>MVGYSSKLIFVSMITRHGDRAPFANIENANYSWGTELSELTPIGMNQEYNLGLQLRKRYIDKFGLLPEHYVDQSIYVLSSHTNRTVVSAQSLLMGLYPAGTGPLIGDGDP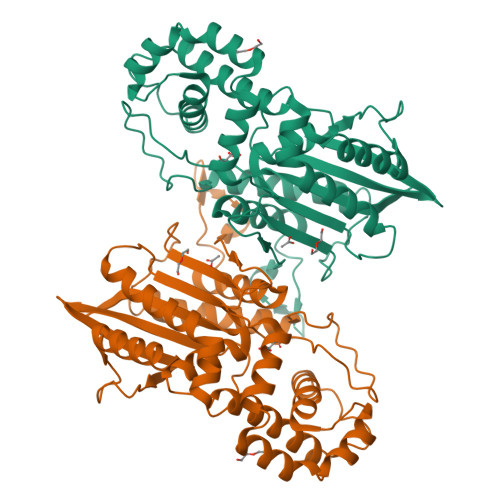AIKDRFQPIPIMTLSADSRLIQFPYEQYLAVLKKYVYNSPEWQNKTKEAAPNFAKWQQILGNRISGLNDVITVGDVLIVAQAHGKPLPKGLSQEDADQIIALTDWGLAQQFKSQKVSYIMGGKLTNRMIEDLNNAVNGKSKYKMTYYSGHDLTLLEVMGTLGVPLDTAPGYASNLEMELYKDGDIYTVKLRYNGKYVKLPIMDKNNSCSLDALNKYMQSINEKFQKHHHHHH[2x]>[4x]CLKLNLLDHVFANPFMNAAGVLCSTEEDLR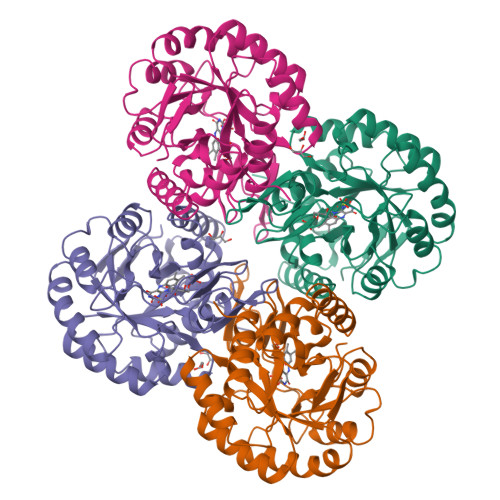CMTASSSGALVSKSCTSAPRDGNPEPRYMAVPLGSINSMGLPNLGFDFYLKYASDLHDYSKKPLFLSISGLSVEENVAMVRRLAPVAQEKGVLLELNLSCPNVPGKPQVAYDFEAMRTYLQQVSLAYGLPFGVKMPPYFDIAHFDTAAAVLNEFPLVKFVTCVNSVGNGLVIDAESESVVIKPKQGFGGLGGKYILPTALANVNAFYRRCPDKLVFGCGGVYSGEDAFLHILAGASMVQVGTALQEEGPGIFTRLEDELLEIMARKGYRTLEEFRGRVKTIE> GPMATESPNSVQKIVVHLRATGGAPILKQSKFKVSGSDKFANV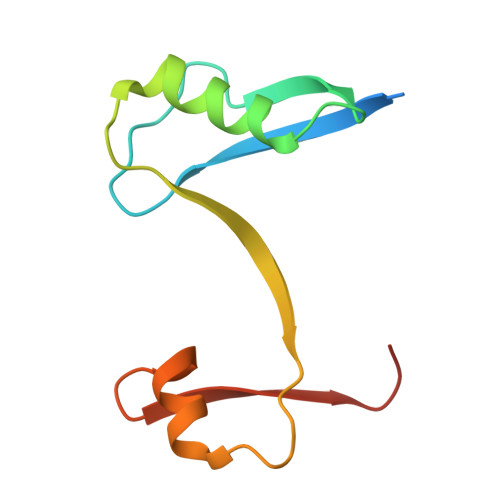IDFLRRQLHSDSLFVYVNSAFSPNPDESVIDLYNNFGFDGKLVVNYACSMAWG> NEILQTLL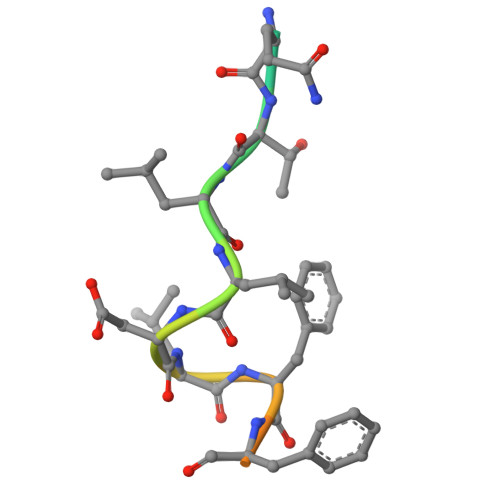DLFFPGYSK> HHHHHHSSGENLYEQGHMPPWTARQDSTTGLYAPVTPAGRVLLDRLAAHLPRIRSTAAEHDRDGTFPTDTFDALRKDGLMGATVPAELGGLGVDRLYDVAVALLAVARADASTALALHMQLSRGLTLGYEWRHGDERARTLAERILRGMVAGDAVVCSGIKDHHTAVTTLRPDGAGGWLLSGRKTLVSMAPVGTHFVINARTDGTDGPPRLASPVVTRDTPGFTVLDN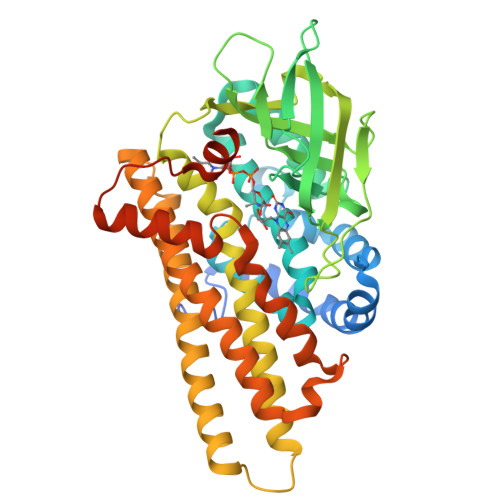WDGLGMRASGTVDIVFDDCPIPADHVLMRDPVGARNDAVLAGQTVSSVSVLGVYVGVAQAAYDTAVAALERRPEPPQAAALTLVAEIDSRLYALRATAGSALTAADALSADLSGDMDERGRQMMRHFQCAKLAVNRLAPEIVSDCLSLVGGASYTAGHPLARLLRDVQAGRFMQPYAYVDAVDFLSAQALGIERDNNYMSTWAKRSGGNGKSADAAGPRRPTPTSR(1P)-N-(5-tert-butyl-2-{[(3S)-hexan-3-yl]oxy}phenyl)-1-(2,5-dimethoxyphenyl)-5-methyl-1H-1,2,3-triazole-4-carboxamide 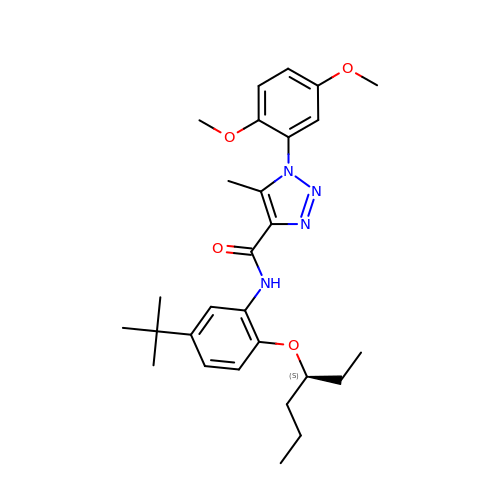| C28 H38 N4 O4 | HPFQSDGKIYUBEE-FQEVSTJZSA-N> VTVIPREQHAISRKDISENALKVMYRLNKAGYEAWLVGGGVRDLLLGKKPKDFDVTTNATPEQVRKLFRNCRLVGRRFRLAHVMFGPEIIEVATFRGHHEGNVSDRTTSQRGQNGMLLRDNIFGSIEEDAQRRDFTINSLYYSVADFTVRDYVGGMKDLKDGVIRLIGNPETRYREDPVRMLRAVRFAAKLGMRISPETAEPIPRLATLLNDIPPAHLFEESLKLLQAGYGYETYKLLCEYHLFQPLFPTITRYFTENGDSPMERIIEQVLKNTDTRIHNDMRVNPAFLFAAMFWYPLLETAQKIAQESGLTYHDAFALAMNDVLDEACRSLAIPKRLTTLTRDIWQLQLRMSRRQGKRAWKLLEHPKFRAAYDL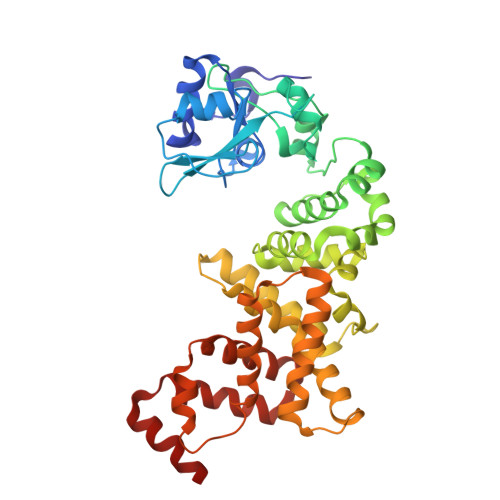LALRAEVERNAELQRLVKWWGEFQVSAPPDQKGMLNELD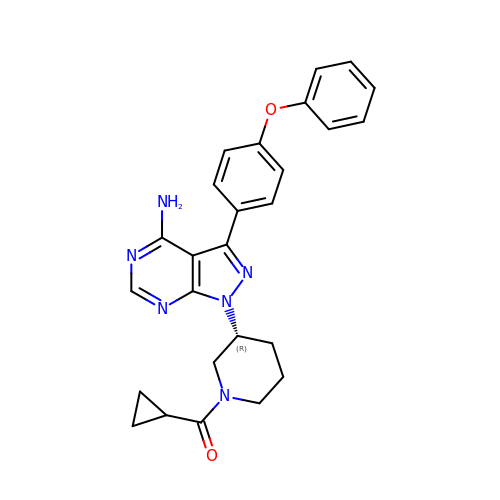{(3R)-3-[4-amino-3-(4-phenoxyphenyl)-1H-pyrazolo[3,4-d]pyrimidin-1-yl]piperidin-1-yl}(cyclopropyl)methanone | C26 H26 N6 O2 | GMAYFNOHSBTWNT-LJQANCHMSA-N>[2x]GAMPHDPSFTPTQLAARAAYLLRGNDLGTMTTAAPLLYPHMWSWDAAFVAIGLAPLSVERAVVELDTLLSAQWRNGMIPHIVFANGVDGYFPGPARWATATLADNAPRNRLTSGITQPPVHAIAVQRILEHARTRGRSTRAVAEAFLDRRWGDLMRWHRWLAECRDRNERGRITLYHGWESGMDNSPRWDSAYANVVPGKLPEYQRADNVIITDPSQRPSDGEYDRYLWLLEEMKAVRYDDERLPSVMSFQVEDVFFSAIFSVACQVLAEIGEDYKRPHADVKDLYLWAERFRAGVVETTDQRTGAARDFDVLAEKWLVTETAAQFAPLLCGGLPHDRERALLKLLEGPRFCGHPDLKYGLIPSTSPVSRDFRPREYWRGPVWPVLTWLFSWCFARRGWAERARLLRQEGLRQASDGSFAAYYEPFTGEPLGSMQQSWTAAAVLDWLG

A glucosylglycerate hydrolase (GgH) identified in M. hassiacum and found to be highly conserved among rapidly growing mycobacteria is likely to be responsible for the rapid mobilization of GG accumulated during nitrogen starvation by hydrolysing it to glucose and glycerate. The MhGgH monomer displays an (α/α)6-barrel domain typical of glycoside hydrolase family 63 (GH63), to which MhGgH belongs. While the active site of GH63 members acting on larger substrates is located in an open, solvent-accessible cleft, those of MhGgH and of MgH from T. thermophilus are covered by a cap domain (subdivided into A′- and B′-regions) with constrained access through a narrow negatively charged tunnel. The crystallographic structure of MhGgH revealed a homotetrameric architecture, which is compatible with the oligomeric organization of the enzyme in solution as assessed by SAXS.

MhGgH was unable to hydrolyse GGlycerol and GGlycolate, despite their considerable similarity to GG. The structures of the E419A variant in complex with both compounds and that of the D182A variant in complex with GGlycolate were determined and help in understanding this behaviour. The most significant differences from the complexes with GG/MG are observed at subsite +1. In the E419A–GGlycerol complex the glycerol moiety of the ligand is stabilized by a direct polar contact with Trp40 and by water-mediated contacts with Tyr88, Gln115, Trp177, Asp182 and Tyr222. In particular, interactions with Tyr36, a key residue for active-site closure and organization, are always absent, while different subsets of interactions are observed for GGlycerol and GGlycolate. Any deviation from these strict interaction patterns will result in a decreased affinity for and highly reduced activity towards the compound, as observed for GGlycerol and GGlycolate. The structures of catalytically inactive variants of MhGgH in complex with these substrate analogues were determined, revealing the important contribution of the reducing end of the substrate to active-site closure and the ensuing enzymatic processing.> MEEDLEDEQIKEASSQLLATHISDEQLKRPLRDYGEALEMWSTFQTKTQALSQSLSSQLRLILTPTQSTKLSGAFRTGKRLNIKKIIPYIASSYKRDKIWMRRAIPSKRAYQILLCVDDSSSMSDDNRSTAGNLALESLVMVARALTVLEAGQIGVMGFGTDVFVAHALTDPPFTSQDAGARVLQQFTFRQDSTDMVLLLRRTIDHFREARLIQASSSRGGEDLWQLALILSDGLVQSRDHARLRPLLREAMEQRVMVVFIVMDDARSRKGHSVLELKEARFGPD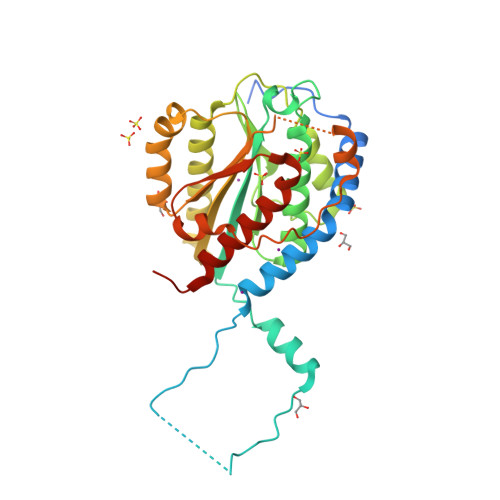GVPVIHRYLDSFPFPYYLIVHHLEDLPGALAALLRTWFAEVNSGSHHHHHH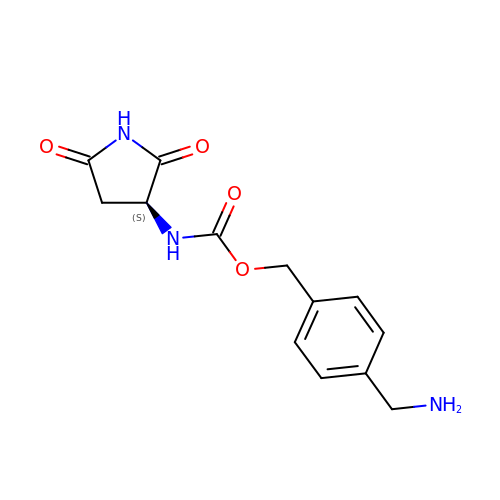[4-(aminomethyl)phenyl]methyl ~{N}-[(3~{S})-2,5-bis(oxidanylidene)pyrrolidin-3-yl]carbamate | C13 H15 N3 O4 | PPHDAIUDWPTCMT-JTQLQIEISA-N> AAMVTQRFVELGWIDSTSPVNEQITNPALVEQIYHSNNDQLLWSDLATANHFEAQLEVIHRASFSPLFSRQLFALKSYRQQDRWHEYDVLATDTLLQYLSYAEQAPKVGIAWFFEGQLDQPLAPPSEEAQLALHMAIGNQSLARLMDEYTPQDPAYQQLLQAYQSLSSIEFNEVALYEQMERLKRPGDPLSHREALVQRLALVNLDTTSILNDVAYYDASLEKPIKQFQKMHGLQTDGVIGPQTMKWLNTSVTERLALLALNAERIRLWPTQQDSMIVVNVPGFDMKYWDAGREVFESKVVVGKTTRPTPVMNTKLDSLIINPTWNVPHKI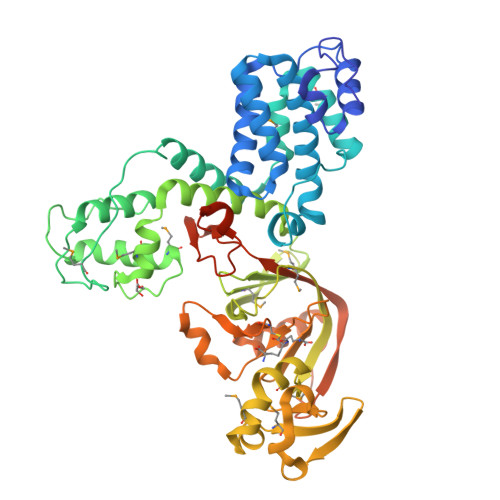MVEDILPMVKRDSEYLANHHMEIIRGWSDPEVIDPALIDWEAVEPETFPYRLRQQAGVQNALGTYKFNTPNSRAIYLHDTPSKHLFNNASRAFSSGCIRVENAEKFAQTLLANQGITLDDFPVSTQAIALKKRIPVHIIYQTVWYEEGVLHYRDDIYHYDALALGNGDASPNLTKIENLYFQGSSSHHHHHH> MAWDLKVKMLGGNDFLVSVTNSMTVSELKKQIAQKIGVPAFQQRLAHQTAVLQDGLTLSSLGLGPSSTVMLVVQNCSEPLSILVRNERGHSNIYE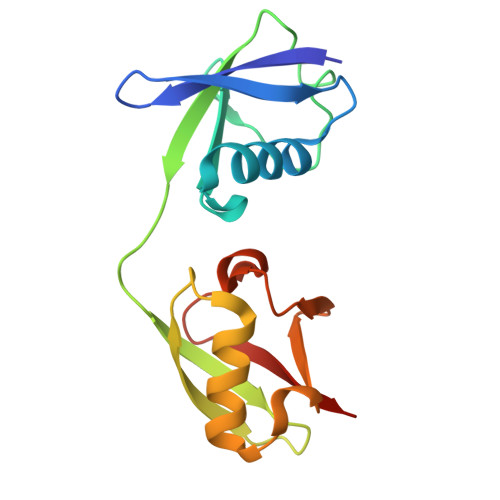VFLTQTVDTLKKKVSQREQVHEDQFWLSFEGRPMEDKELLGEYGLKPQCTVIKHLRLR>GMERILKKQPAPVRALTIHPLRRYESSIYDTPIPAYVIKHSSDGVTIDIATSELADGQSGSTIQPFESVPAQNLTLFKHDFTFGHLADTTDKKFVEVFGVLENRADDSDFQSPDMIIETETGHVYVVEFTTTMGDANSADLAARNKIAK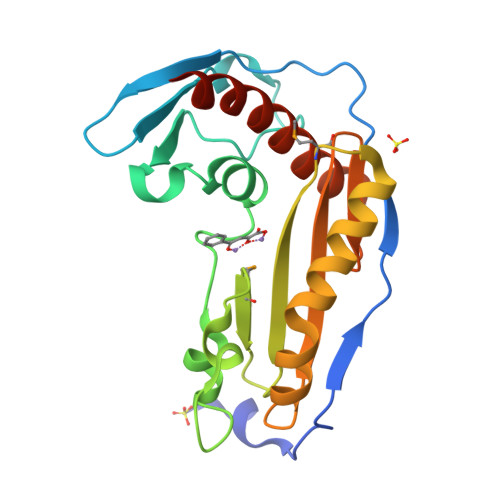YEIACLDRSAIKPISLYIIAVHFNGVVSNLDLSDEEVNEIVFRFRLARDIFEELREINPALFD[2x]> VTKVISQASPVPTSIPGVADLVGFGTGGVYIIRNSLLVQVVKVINNFGYDAGGWRTEKHVRLLADTTGDNQSDVVGFGEDGVWISTNNGDNTFTDPPSHVLANFSYLAGGWRVEKHIRFMADMRKTGRADIVGFGEAGILISRNNGSSQFAPTQLALNDFAYAQGWRLDRHLRFLGDITGNGLLDVVGFGENHVFVAKNNGNGTFQPAQAVVNNFCVGAGGWTIASHPRVIADLTGDSRADILGFGGAGVYTSLNNGNGTFGAVNLVLMDFGVASGWRTAKHVRCVAPLTSKKVGDIIGFGDAGVYVALNNGDGTFGPVKRVINNFGYNQGWRVDKHPRFVV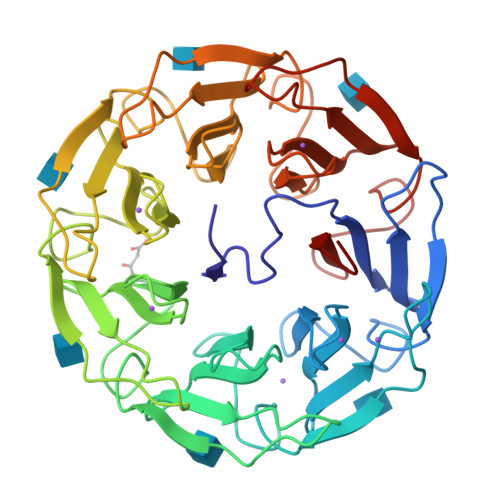DLTGDGAADIVGFGENSTWACMNKGDGTFGPDMKLISDDTSSKGWTLEKTVRYAANLYA> MSLVNRKQLEKMANVRFRTQEDEYVAILDALEEYHNMSENTVVEKYLKLKDINSLTDICIDTYKKSGRNKALKKFKEYLVTEVLELKNNNLTPVEKNLHFVWIGGQINDTAINYINQWKDVNSDYNVNVFYDSNAFLINTLKKTVVESAINDTLESFRENLNDPRFDYNKFFRKRMEIIYDKQKNFINYYKAQREENPELIIDDIVKTYLSNEYSKEIDELNTYIEESLNKITQNSGNDVRNFGEFKNGESFNLYEQELVERWNLAAASDILRISALKEIGGMYLDVDMLPGIQPDLFESIEKPSSVTVDFWEMTKLEAIMKYKEYIPEYTSEHFDMLDEEVQSSFESVLASKSDKSEIFSSLGDMEA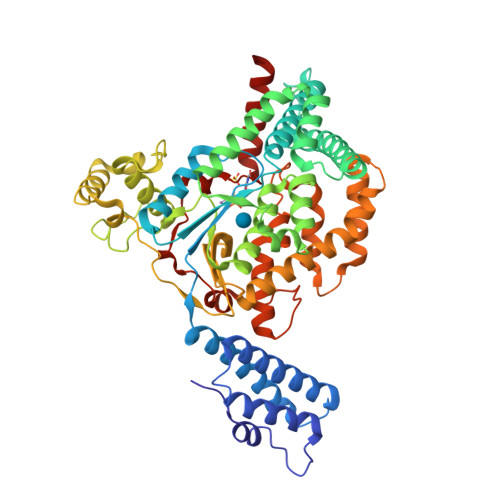SPLEVKIAFNSKGIINQGLISVKDSYCSNLIVKQIENRYKILNNSLNPAISEDNDFNTTTNTFIDSIMAEANADNGRFMMELGKYLRVGFFPDVKTTINLSGPEAYAAAYQDLLMFKEGSMNIHLIEADLRNFEISKTNISQSTEQEMASLWSFDDARAKAQFEEYKRNYFEGA>MTHHYPTDDIKIKEVKELLPPIAHLYELPISKEASGLVHRTRQEISDLVHGRDKRLLVIIGPCSIHDPKAALEYAERLLKLRKQYENELLIVMRVYFEKPRTTVGWKGLINDPHLDGTFDINFGLRQARSLLLSLNNMGMPASTEF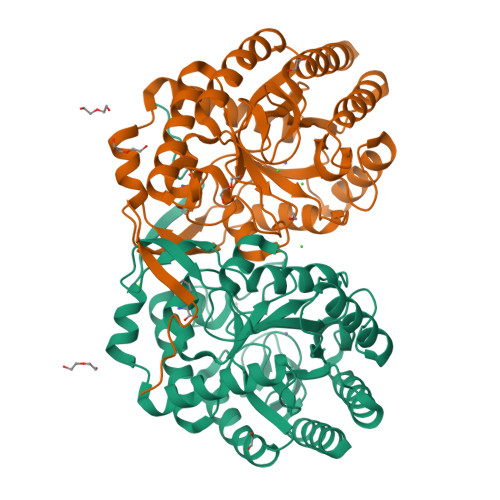LDMITPQYYADLISWGAIGARTTESQVHRELASGLSCPVGFKNGTDGNLKIAIDAIGAASHSHHFLSVTKAGHSAIAHTGGNPDCHVILRGGKEPNYDAEHVSEAAEQLRAAGVTDKLMIDCSHANSRKDYTRQMEVAQDIAAQLEQDGGNIMGVMVESHLVEGRQDKPEVYGKSITDACIGWGATEELLALLAGANKKRMARAS[2x]> MGSSHHHHHHSQDPNSMTTLTRQDLNFGQVVADVLCEFLEVAVHLILYVREVYPVGIFQKRKKYNVPVQMSCHPELNQYIQDTLHCVKPLLEKNDVEKVVVVILDKEHRPVEKFVFEITQPPLLSISSDSLLSHVEQLLAAFILKISVCDAVLDHNPPGCTFTVLVHTREAATRNMEKIQVIKDFPWILADEQDVHMHDPRLIPLKTMTSDILKMQLYVEERAHKGS;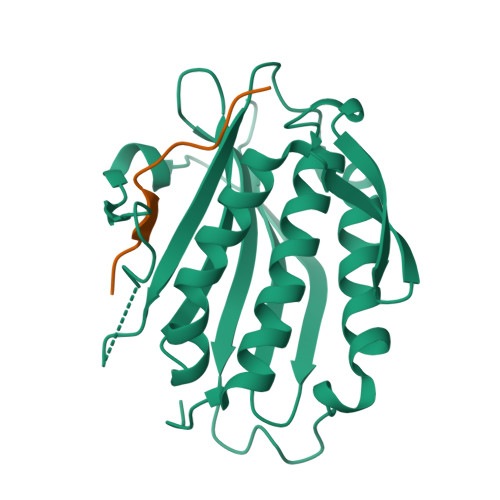> MSNPSASSGPWKPAKPAPSVS N-[6-(4-amino-1-{[2-(4-methylpiperazin-1-yl)quinolin-3-yl]methyl}-1H-pyrazolo[3,4-d]pyrimidin-3-yl)-1,3-benzothiazol-2-yl]acetamide 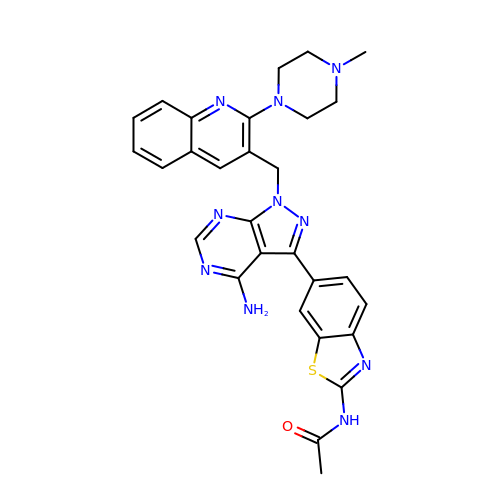| C29 H28 N10 O S | PROYLAOFEKHQGS-UHFFFAOYSA-N>[2x]MSEQLVTPENVTTKDGKINLLDLNRQQMREFFKDLGEKPFRADQVMKWMYHYCCDNFDEMTDINKVLRGKLKEVAEIRAPEVVEEQRSSD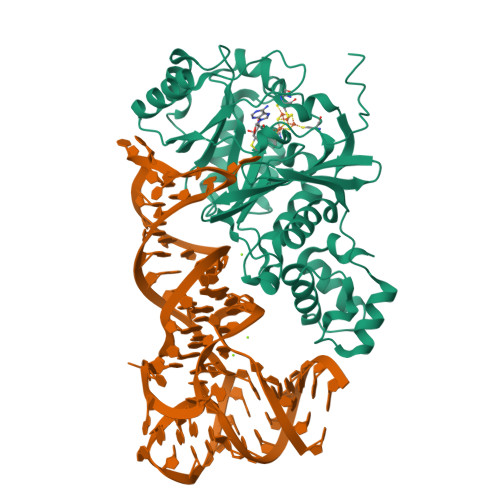GTIKWAIAVGDQRVETVYIPEDDRATLAVSSQVGCALECKFCSTAQQGFNRNLRVSEIIGQVWRAAKIVGAAKVTGQRPITNVVMMGMGEPLLNLNNVVPAMEIMLDDFGFGLSKRRVTLSTSGVVPALDKLGDMIDVALAISLHAPNDEIRDEIVPINKKYNIETFLAAVRRYLEKSNANQGRVTIEYVMLDHVNDGTEHAHQLAELLKDTPCKINLIPWNPFPGAPYGRSSNSRIDRFSKVLMSYGFTTIVRKTRGDDIDAACGQLAGDVIDRTKRTLRKRMQGEAIDIKAVGNSSSVDKLAAALEHHHHHH FNR is a flavoenzyme that contains a noncovalently bound flavin adenine dinucleotide (FAD) as a prosthetic group. It catalyzes redox reactions between Fd and NAD(P)H. The redox-active component is the isoalloxazine ring of FAD, which undergoes transitions among three states: fully oxidized (FAD), semiquinone (; partially reduced) and hydroquinone (FADH2; fully reduced). In root plastids, which lack PS I, R-FNR reduces nonphotosynthetic Fd by oxidizing NADPH from the oxidative pentose phosphate pathway.

The structure of R115A mutant FNR (mtFNR) was also determined in the oxidized form (mtFNRoxi) to examine the arrangement of water molecules around the FAD moiety. Although the space group of the mtFNRoxi crystals differed (P3121), the main-chain structure of mtFNRoxi was highly similar to those of wtFNRoxi and wtFNRred. Focusing on the water molecules surrounding FAD, the arrangement in the mtFNRoxi structure closely resembled that in wtFNRred. The R115A mutant (mtFNR) mimicked the dis­ordered side chain of wtFNRred, with its X-ray structure confirming that the water-molecule positions in mtFNRoxi resemble those in wtFNRred.

> SKVSVAPLHLESAKEPPLNTYKPKEPFTATIVSVESLVGPKAPGETCHIVIDHGGNVPYWEGQSYGVIPPGENPKKPGAPQNVRLYSIASTRYGDNFDGRTGSLCVARAVYYDPETGKEDPSKNGVCSNFLCNSKPGDKIQLTGPSGKIMLLPEEDPNATHIMIATGTGVAPFRGYLRRMFMEDVPNYRFGGLAWLFLGVANSDSLLYDEEFTSYLKQYPDNFRYDKALSREQKNRSGGKMYVQDKIEEYSDEIFKLLDGGAHIYFCGLKGMMPGIQDTLKKVAERRGESWDQKLAQLKKNKQWHVEVY> MLKQPIQAQQLIELLKVHYGIDIHTAQFIQGGADTNAFAYQADSESKSYFIKLKYGYHDEINLSI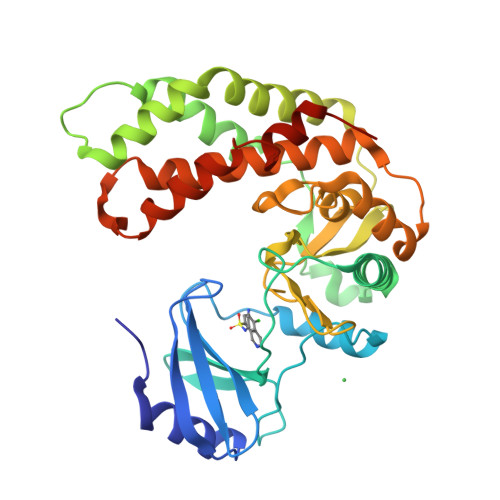IRLLHDSGIKEIIFPIHTLEAKLFQQLKHFKIIAYPFIHAPNGFTQNLTGKQWKQLGKVLRQIHETSVPISIQQQLRKEIYSPKWREIVRSFYNQIEFDNSDDKLTAAFKSFFNQNSAAIHRLVDTSEKLSKKIQPDLDKYVLCHSDIHAGNVLVGNEESIYIIDWDEPMLAPKERDLMFIGGGVGNVWNKPHEIQYFYEGYGEINVDKTILSYYRHERIVEDIAVYGQDLLSRNQNNQSRLESFKYFKEMFDPNNVVEIAFATEQLEHHHHHH>FTLIELMIVVAIIGILAAIAIPQYQNYVARSEGASALATINPLKTTVEESLSRGIAGSKIKIGTTASTATETYVGVEPDANKLGVIAVAIEDSGAGDITFTFQTGTSSPKNATKVIT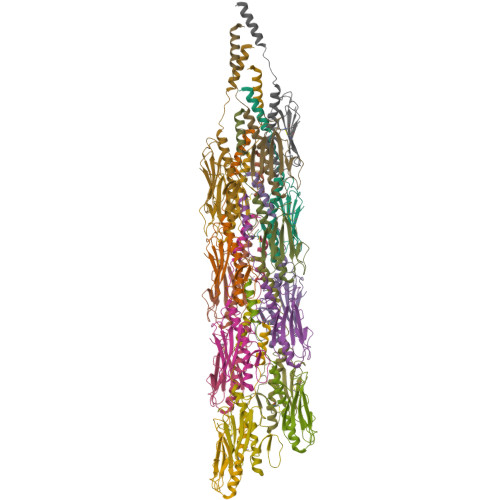LNRTADGVWACKSTQDPMFTPKGCDN[16x]> MASDMEEKFREAFILFSSCSDHIEMYKFFELMNSFGIILTNDEKAALPNDINMDYWLNFAKKHYNYEQPFKHINNVNEQNTN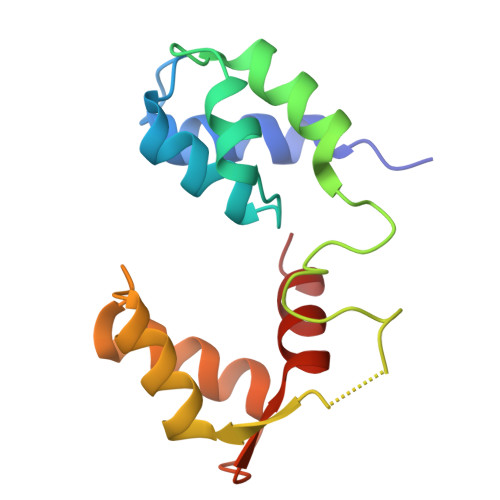VQIKIDNFLGIMKALDTRLTESDLNILLQITNPENKSTLNLKTVSQKLTESI> PNFSGNWKIIRSENFEELLKVLGVNVMLRKIAVAAASKYAVEIKQEGDTFYIKVSTTVYTTEINFKVGEEFEEQTVDG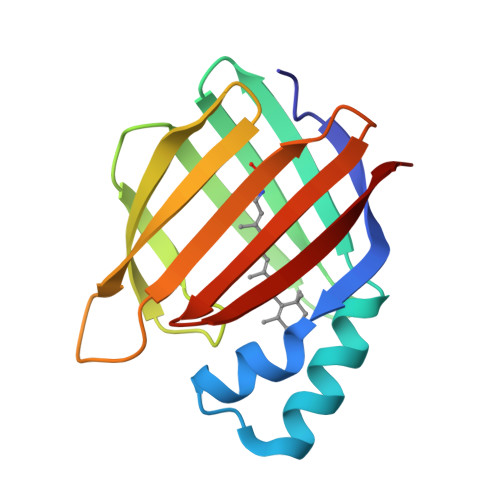RPCKSLVKWESENKMVCEQKLLKGEGPKTSWTKELTNDGELIMTMTADDVVCTQVFVRE>MKLRASVLIGATILCLILSACSNYAKKVVKQKNHVYTPVYNELIEKYSEIPLNDKLKDTPFMVQVKLPNYKDYLLDNKQVVLTFKLVHHSKKITLIGDANKILQYKNYFQANGARSDIDFYLQPTLNQKGVVMIASNYNDNPNSKEKPQTF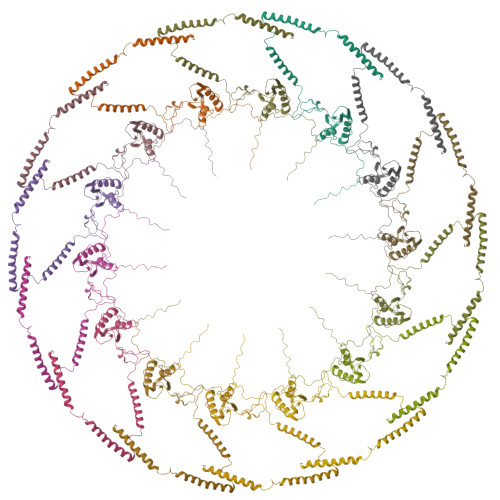DVLQGSQPMLGANTKNLHGYDVSGANNKQVINEVAREKAQLEKINQYYKTLLQDKEQEYTTRKNNQREILETLSNRAGYQMRQNVISSEIFKNGNLNMQAKEEEVREKLQEERENEYLRNQIRSLLSGK[14x]> DISEPPLHDFYCSRLLDLVFLLDGSSRLSEAEFEVLKAFVVDMMERLRISQKWVRVAVVEYHDGSHAYIGLKDRKRPSELRRIASQVKYAGSQVASTSEVLKYTLFQIFSKIDRPEASRIALLLMASQEPQRMSRNFVRYVQGLKKKKVIVIPVGIGPHANLKQIRLIEKQAPENKAFVLSSVDELEQQRDEIVSYLCDLAPEAPPPT;> DCPSGWSSYEGNCYKFFQQKMNWADAERFCSEQAKGGHLVSIKIYSKEKDFVGDLVTKNIQSSDLYAWIGLRVENKEKQCSSEWSDGSSVSYENVVERTVKKCFALEKDLGFVLWINLYCAQKNPFVCKSPPP;> DCPPDWSSYEGHCYRFFKEWMHWDDAEEFCTEQQTGAHLVSFQSKEEADFVRSLTSEMLKGDVVWIGLSDVWNKCRFEWTDGMEFDYDDYYLIAEYECVASKPTNNKWWIIPCTRFKNFVCEFQA;> HPICEVSKVASHLEVNCDKRQLTALPPDLPKDTTILHLSENLLYTFSLATLMPYTRLTQLNLDRCELTKLQVDGTLPVLGTLD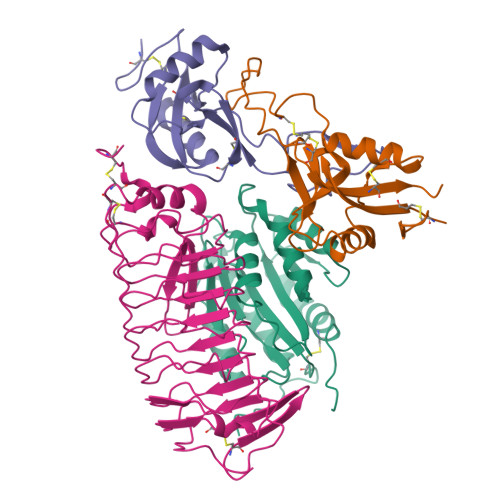LSHNQLQSLPLLGQTLPALTVLDVSFNRLTSLPLGALRGLGELQELYLKGNELKTLPPGLLTPTPKLEKLSLANNQLTELPAGLLNGLENLDTLLLQENSLYTIPKGFFGSHLLPFAFLHGNPWLCNCEILYFRRWLQDNAENVYVWKQGVDVKAMTSNVASVQCDNSDKFPVYKYPGKGCP>GDGTKVEELNKATAAMMVPFDSVKFTGNYGNMTEISYQVAKRAAKKGAKYYHITRQWQERGNNITISADL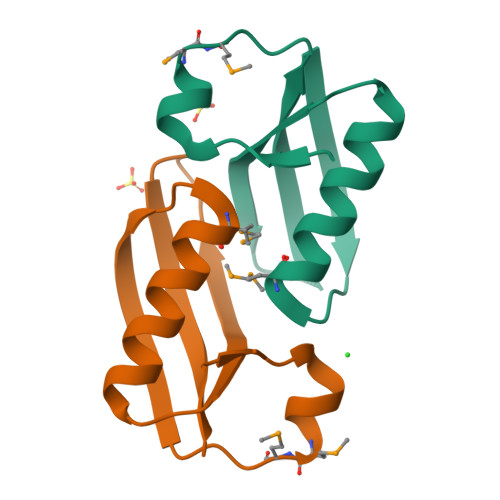YK[2x]>GPLGSMASPEERLLDELNNVIVSFLCDSGSLEVERCSGAHVFSRGSSQPLCTVKLRHGQIYHLEFVYKFLAFKLKNCNYPSSPVFVISNNGLATTLRCFLHEPSGLRSGQSGPCLGLSTDVDLPKNSIIMLGQDDFIKFKSPLVFPAELDLLKSMVVCRAYITEHRTTMQFLVFQAANAQKASRVMDMISDMSQQLSRSG[5x];>[5x]GPGSRSICSRHTRHGVDRSHFSLRDFFRGISANFELGKDFLREMNTPIHVSEAVFLPLSLCTLSPGRCLRLSPFGHSLTLGSHCEICINRSQVHVPQEFSSTQLSFFNNVHKIIPNKTFYVSLLSSSPSAVKAGLSQPSLLYAYLVTGHFCGTICPIFSTNGKGRLIMHLLLQGTSLHIPETCLKLLCENIGPTYELAVDLVGDAFCIKVSPRDTVYEKAVNVDEDAIYEAIKDLECGDELRLQII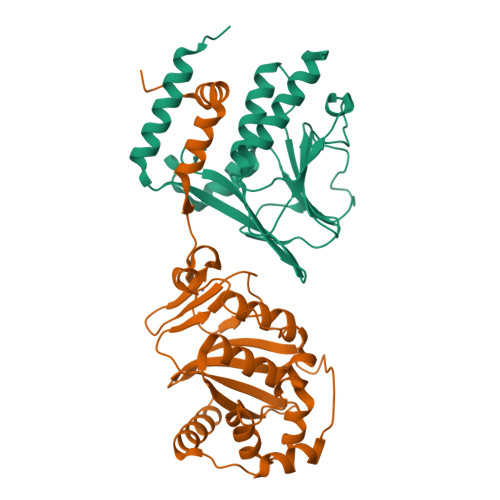NYTQLILENKQ>[2x]MNHKVHHHHHHIEGRHMTTAQHPTDEDLLARVLVPYKDHCKYLRSAVVTESDTGRAVARCEFAIPESCYIDDTGHLNSVEVNICYNQMMYYLVA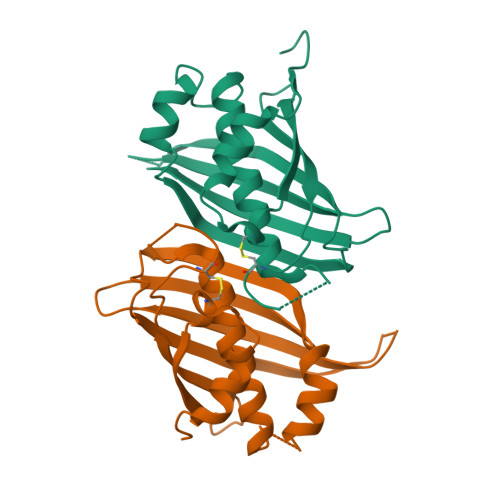KSVKEGLLAGFESWTLDDFWKHQLPDILIARFASNFRRPVNPRAFSGEMEFQSVTRRAPAGGIPFLHAETAYRYWDADSGRCDGEAVLAFVNIP> GGAAUUAGAGUGUGUUCCUGAACUGCUUCGGCGGUUCGCUACGUUCUUCGGAAUGUAUAUAGUGUUCGCAUUAUACCGUAGUCCAAGCCGUGUGGUUCGCCGCACGUCGUUCGUUCGCGGACGAGCAGGUGCCAUAACCUCCAAAUGGUACCUGCGCGUGUUGUCAGCAAGGUCUAAGCUGAUAACACUAUGCUAACGACUGAAGCAUAUUGGAUUACGGGCCAAGGGCAGCUAAGAUCGGAAGCUGUCCUUGAGGAACGCACUCUGAUUCCCCUCCGGAAGGAGCCCCACAGGUAAUAAACCGAUCAUAUUACUUGUGCACUCGCAACAGUCGAGCGGGUGGUAAUGAUUGCGCCCGUUGGCUAGAAUAGACCACUAGCUAACGGCGGGUCUUGGAUCAAUGGAGGAGAUCCAGGACCCGACCCGGACUU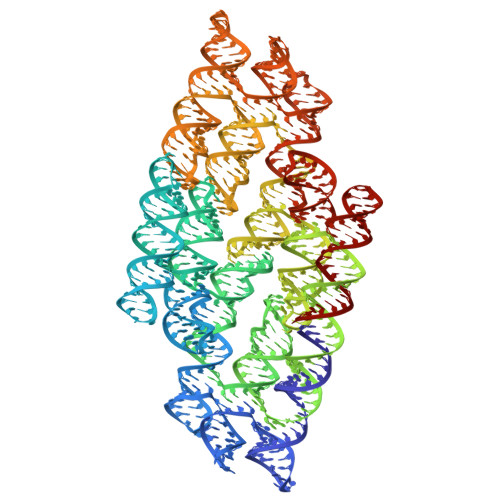CGGUUCGGGUGCGGCCUUAGUUCGCUGAGGCCCGUCGCAUUCGUGUGACGGUGGUUAUUGCGGUCAAGGUUUCGACUUUGAGUAUUCCUUCGGGGAUACGCUUCUUCUGGAGG(1R)-N-(4-tert-butyl-3-fluorophenyl)-6-methoxy-2-[(3-oxo-2,3-dihydro-1,2-oxazol-5-yl)acetyl]-1,2,3,4-tetrahydroisoquinoline-1-carboxamide 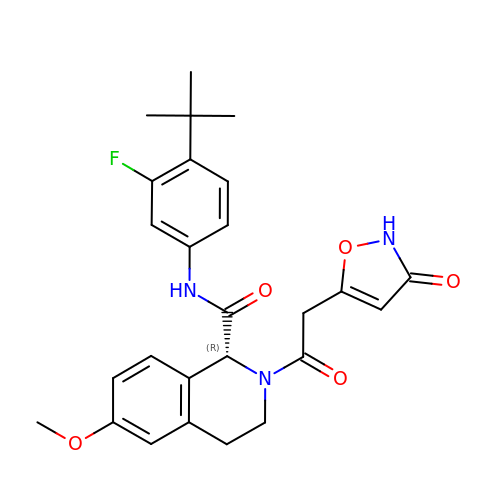| C26 H28 F N3 O5 | GSZJCGDGBYIJKI-XMMPIXPASA-N> PEAEGPTVE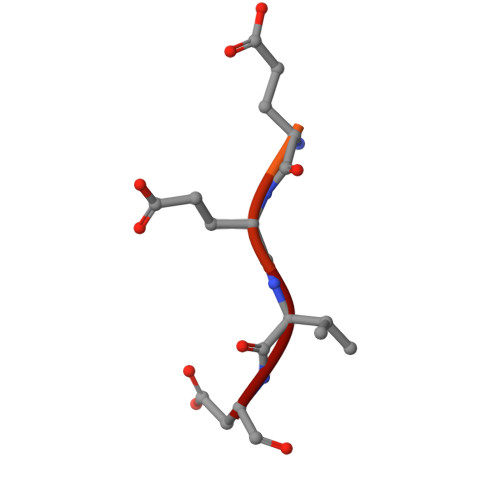EVD>[2x]GAMESTVNALTSE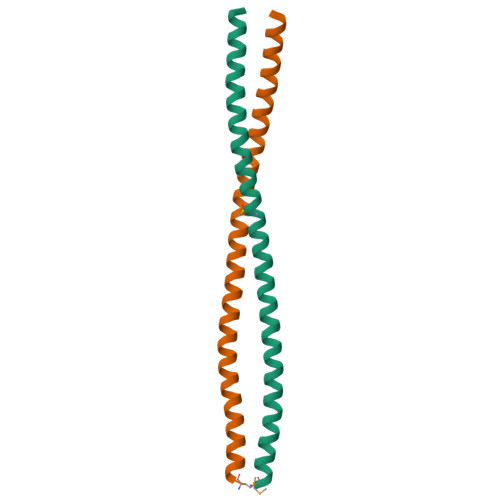LRDLRAQREEAAAAHAQEVRRLQEQARDLGKQRDSCLREAEELRTQLRLLEDARDGLRRELLEAQRKLRESQEGREVQRQEAGEW> GNLVPFTKNAFKDWCSVNGKRLIILALEISSAVSNSRGNSAGSTSGKVNVIDPSGLVRLLSDLVESQDTFVYLLSYLQRSDLDIMFKRYPQIGLIAENGNFVKLIGAKNWISLADKDELNSWMPEIVKLVESKVERLPGSFCEALDATVRFHAGKSFSEDRERSLDTMGETIQHINTLFEHNGVHATLVRNSVIVQKDQISLKAIRLVLSCHNSN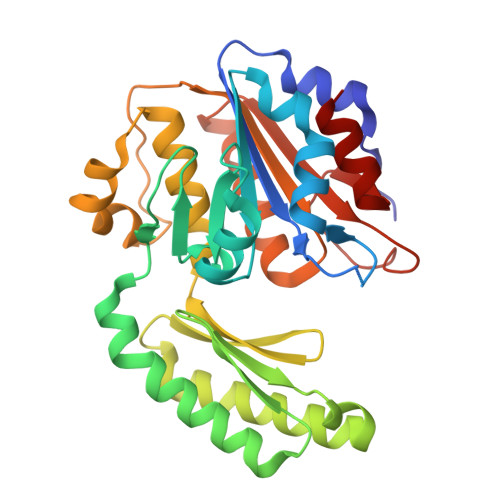LDQKYVVTHINEFQQPMKDDIPSNDHEVAAVLYSGGLTSIDEANYEYVNSLKKDIGNTLTVTLISSSNEETKTAATYGVRGINELLCILNS> GSPSRSVKLAGNSSLCPVSGWAIYSKDNSVRIGSKGDVFVIREPFISCSPLECRTFFLTQGALLNDKHSNGTIKDRSPYRTLMSCPIGEVPSPYNSRFESVAWSASACHDGINWLTIGISGPDSGAVAVLKYNGIITDTIKSWRNNILRTQESECACVNGSCFTIMTDGPSDGQASYKIFRIEKGKIIKSVEMKAPNYHYEECSCYPDSSEITCVCRDNWHGSNRPWVSFNQNLEYQMGYICSGVFGDNPRPNDKTGSCGPVSSNGANGVKGFSFKYGNGVWIGRTKSISSRKGFEMIWDPNGWTGTDNKFSIKQDIVGINEWSGYSGSFVQHPELTGLDCIRPCFWVELIRGRPEENTIWTSGSSISFCGVNSDTVGWSWPDGAELPFTIDK

The NA is a homotetramer and is classified as a type 2 membrane protein. Each monomer consists of a cytoplasmic tail, a transmembrane domain, a hypervariable stalk domain, and a globular head domain. The globular head domain of each monomer contains an enzymatic active site, whose activity plays an integral role during the viral replication cycle. In particular, the NA cleaves sialic acid residues from newly formed virions as they bud from the viral host cell surface.

Here, we generated stable soluble recombinant NA constructs of the N1 subtype (A/Michigan/45/15 H1N1 [Mich15] strain) using the baculovirus expression system. The constructs were engineered to contain either a measles virus phosphoprotein tetramerization domain (N1-MPP), a Sendai virus phosphoprotein tetramerization domain (N1-SPP), or a leucine zipper from the SEPPALLATA-like MADS domain transcription factor derived from Arabidopsis thaliana (N1-SEP). The measles virus tetramerization domain-based construct, termed N1-MPP, was chosen for further evaluation, as it retained antigenicity, neuraminidase activity, and structural integrity and provided robust protection in vivo against lethal virus challenge in the mouse model. N1 NA expressed as N1-MPP resembles previously solved N1 NA structures. To verify the correct conformation of the N1 NA head domain (residues 82 to 471, N2 numbering) from A/Michigan/45/2015 (H1N1) in the recombinant N1-MPP, the N1-MPP was first expressed in Sf9 insect cells and purified, and the N1 head was obtained by removing the MPP tetramerization domain from N1-MPP with thrombin. The crystal structure of the N1 NA head was determined to a 2.90-Å resolution. The overall structure shows a typical box-shaped tetramer and resembles other published N1 structures, such as the N1 NA head from A/California/04/2009 (H1N1), with a root mean square deviation (RMSD) value of 0.28 Å for all Cα atoms. Ten residues that are different between A/Michigan/45/2015 and A/California/04/2009 (H1N1) are located over the outer region of the head domain, where residues 199, 247, 263, 269, 314, 372, 389, and 432 are solvent exposed and residues 240 and 321 are buried but have similar hydrophobic residues. N1 NA expressed with this tetramerization domain was intact and resembled structures of N1 NA that were previously solved. N1-MPP and N1-SPP exhibited high enzymatic activity, comparable to that of the positive control, N1-VASP, which indicates correct folding of the proteins.> MRSSKSPFKRKSHSRETSHDENTSFFHKRTISGSSAHHSRNVSQGAVPSSAPPVSGGNYSHKRNVSRASNSSQTSNFLAEQYERDRKAIINCCFSRPDHKTGEPPNNYITHVRIIEDSKFPSSRPPPDSKLENKKKRLLILSAKPNNAKLIQIHKARENSDGSFQIGRTWQLTELVRVEKDLEISEGFILTMSKKYYWETNSAKERTVFIKSLITLYIQTFEGHVPELVNWDLSLFYLDERSYQRAVITNRPGSVSPIKSPTSNFTTNTTQSVGSVPFSAPTERTRRSETESVNPVSTPASVEYHAGMKSLNKAPYSSNSTLNEVNKRYELEQQQQQEEAELRRLEEQKRLQLQKENEMKRLEEERRIKQEERKRQMELEHQRQLEEEERKRQMELEAKKQMELKRQRQFEEEQRLKKERELLEIQRKQREQETAERLKKEEQEALAKKEEEEKSKRNKVDNESYTQEINGKVDNLLEDLNAVLAEETETTPTMQNGTYVPERSTARAHDQLKKPLNIAKVESLGGSDLNDSISLSDEIAGLNTSNLSGEDQDEKNDLSFEKGDEVRYSNNFEGEAPHVYHEVSIIQEEAPAVSQKLILPEENNESEALIESKEEIKTMENIDDEVLLEILTDINWSIEDDADSMIERIDLRLAETEYLFNQNLLSLQKIGPNIRPYEDKVNDECHRIIPTLSLFLMEMSNFSNDIENVESQDNGLQVESANKKLLWNTLDELLKTVSLDEISLNQLLECPIREKNLPWMENQLNLLLKAFQAIGSDGNEVEYNLREISGLKQRLQFYEKVTKIFLNRIVEEMQKKFSNIRGQDISHDQMIRILTTLLIFSPLILFCKEISQKSYQAIVENWNVSIQPVYMELWTKKISQLQGIDTNDEKMNELSLSQLLNEWDTFRKERKTNDINPVFKNSFSLLTECLQTMRQECIVYQNFVEVFFHISSKHNFEEYIKHFNDPDAPPILLDTVKVMQSDREAAVIETQLVSRIFQPIVTRLSSYFVELVKAEPTVAPALTFYLENEIKSLESSNHEFLLSAVTRMYTQIKQVWSDNVEEQVLHFERISNATTNGEILPGILDLPVGLKNSEDLFQFAKRSMDIKDTDEGYESIELMNSSFRKLSIAATRSITHKEVNSSINPNLSDTAALNNDYMETISLLVNSNWLTEMLSMLNFNKDGIFDTSLQNVKKVFDVEKESYASFLLRDTMPKLTAFVYGVSNIIENTNNVNMTNPSRWAAYSRQNLENILLAYTSHEIETLVKRLHTHMVNDFGYHQENAINNVLCDKLWSCIQGQTVSLYLKLYTVIDKHYRGTNIRFTKNDIISAFEEYKNA;> MDRFQIGDEQLLRFYQLKTINPTHSWAQDSSKLNNEEATSNELGVETSFDILKDFKYGNQISIDKESRAYLNDESLSYIRDPLNGQEMSKELQHLPNDSMRLNYLVNSKQFNVKAFLRDMHKQDSFNDLNNSLDRLDSDIQDQSIHLKQLVGKNFTKYVKIKNKLDQIYKEFDEKTNEKNQCDSPKENQINVESLNKKVDEVIRTTTFKLKPLMDNYQKILNYQATKKFIELNKFYFNLPKSLKRCLTNNDFNEFIIEYSKGLTLRRRFNQSSDASQSLVIKRIWTQIENLLVTYKDLIWNSLINSNFNIDQPQETILSLFSKLLNLENFINNNQRESESGNKNTTSSSNENPILRWMSIKMNGFQNELNELSGHMISKIIHSQRLILQNNTNQDKSQGCVELSYYLKINQLFQIISDTGKDSEGLKSTVEPNKVNTISGTSYLNLNCQPSSQGLTDSPTIIEMWLLILKYINDLWKICDQFIEFWEHIEKFLDGTYQNSIINEKRKENILIGDSNIIESYQKSLILKEEQINEVRLKGEEFITSVSQNLISFFTSSQSSLPSSLKDSTGDITRSNKDSGSPLDYGFIPPNCNGLSCLRYLPKIVEPILKFSTELAQLNITTNGITICRNTLSTIINRCVGAISSTKLRDISNFYQLENWQVYETVTFSSKSQDSSKNLTFEYGVTQFPEIVTSFQEVSIKTTRDLLFAYEKLPIINGISVVSYPSKQLLTGIEIQQIISMEAVLEAILKNAAKDKDNPRNSHTILTLTNLQYFRECAFPNILQYFDDAFEWNLASKNLELFSLLSKMESSIFGNYLSDLKINLRDTLEEKFHEINWPMYTSNSFRVGDYIIEALMILIVVHSECFRIGPQLIHKILIETQIFIARYLFEAFKPYVGNLSNDGSLQIIVDLEFFQKVMGPLLEKDTEATLRACLQNCFQNDTNRLQKCINEINPIVSANLKRTAIQFAAFS;> MSSDPLQQVCDLIKGDLSLERVRDIKEQLLKEKSVVEYQLNKESDKYYGEVEESLKLLNLSKNSVTSIKQQINEVNKLGNDNRFAINRYDILFRATKLYETVNTTSSIYDRIYNFVALMEHIERLLVAELAEDALETGCPHLLEIHFLLTSARDFQEQVVVMAKEATEDAQRTVMKLFSRLSGIISKFDKLLDGLTYDIVEMARAEQISLAIRLFKIYDLEEREDLRIEAIRNIIKKKEIEIEKSSIKKLPNSKNTARLQDETPKVIEYPTNKGLYQEIMSGTISTRTAPRGYKHFLINGINNSISEMFGEMREKYVGDQKFDVLDNMDWIFNELIIVKEHIANCCPPHWNIFEVYFDQYYKELHSLITDLVESEPETIIILDILAFDKTFQDTLKQDFGFTKSEVKSVIGDKEKETLFKDYLNLIVVKMTEWIGNLEKAEFDVFLERSTPPHSDSDGLLFLDGTKTCFQMFTQQVEVAAGTNQAKILVGVVERFSDLLTKRQKNWISKISEEIKKQINYNHKYDIDPESITPEDECPGGLVEYLIAVSNDQMKAADYAVAISSKYGKLVSKVYEKQITNHLEGTLDGFAEVAQCSSLGLITLMFDDLRKPYQEIFSKTWYMGSQAQQIADTLDEYLLDIKPQMNSVLFVNFIDNVIGETIIKFLTALSFEHSFKNKNNKFLEAMKRDFEIFYQLFVKVLDGNESKDTLITQNFTVMEFFMDLSCEPIDSILDIWQKYLEVYWDSRIDLLVGILKCRKDVSSSERKKIVQQATEMLHEYRRNMEANGVDREPTLMRRFVLEFEKQ;> MDYLKPAQKGRRRGLSINSLSETQQSAMNSSLDHLQNDLNRINLQWNRILSDNTNPLELALAFLDDTSVGLGHRYEEFNQLKSQIGSHLQDVVNEHSQVFNTNVASYGKAVSSIMQAQEQTLNLKNCLKEANEKITTDKGSLQELNDNNLKYTKMIDVLVNIEELLQIPEKIEENIRKENFHQVQILLERGFILMNNKSLKTVEILKPINQQLELQEHLLFNNLIEEIHDIMYSKSNKTNFTRVTNNDIFKIISISHNGFTSLENYLYNIVNIDIMEHSKTINKNLEQFIHDQSLNKGNIMLQENAATQAPLAPSRNQENEGFNRIGFLLKTINNINKLPVAFNIITERAKEEIHNIIVKSTESIRSKHPSLLKMATSLKNDNHFGLPVQDILSIILRECFWEIFLKLLYAIQCHRAIFEMSNILQPTSSAKPAFKFNKIWGKLLDEIELLLVRYINDPELISSNNGSIKPINGATNNAPTLPKRKNPKIFSLEYNIEDNSSVKDQAFELKALLKDIFPGFSVSSNMDLDSIYVKDESFEQDEPLVPPSVFNMKVILDPFLLFTQSTSTIVPSVLTQNTISSLTFFDDYMNKSFLPKIQMTMDYLFTVEVESNNPYALELSDENHNIFKTALDFQRLFYNLLNVFNTANTFREKISYCILDLLNHFYNYYLGLFNSL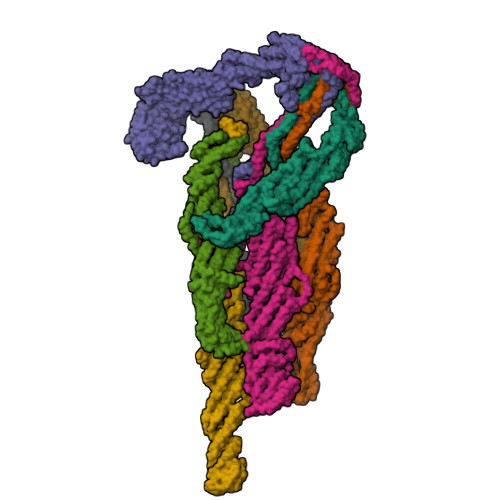IGTSDRHLTRKIITAWLQNGILMDQEQKILNGDETLFHEESIELFKEIPHFYQAGKGLSKSDLFNNLTLDTILQFSASVLWILNWLPGLKKAINIDEVSQEPMLDADRLRSSWTFSESMDLNYSNPSSSPNSLGNLKILLDDKASKKFDETIDGFKTLKFKLITILRFNIRALCIYDIGSFFQNTKIWNMDVGSIELDQNIASLISELRRTESKLKQQLPEKEKNSIFIGLDIVNNYALIKGAKSIKVLNHNGIKKMLRNVNVLQHAYRNLSSEPSKINMNVTMNFYSLCGSSEAELFEYIKDNELPHCSVEDLKTILRLQFSEEMHRQLKRQSTSSTKGSIKPSNKRYTEALEKLSNLEKEQSKEGARTKIGKLKSKLNAVHTANEK;> MNSLYELDPKWKKLLKTDNFLGGLTVNEFVQELSKDHRNDVLIDANTKNLPTNEKDQDAIREAIWKQLDPKPYIRTFESTLKELKNLNEETLNKRQYFSEQVATQEVIHSENVIKLSKDLHTTLLTFDKLDDRLTNVTQVVSPLGDKLETAIKKKQNYIQSVELIRRYNDFYSMGKSDIVEQLRLSKNWKLNLKSVKLMKNLLILSSKLETSSIPKTINTKLVIEKYSEMMENELLENFNSAYRENNFTKLNEIAIILNNFNGGVNVIQSFINQHDYFIDTKQIDLENEFENVFIKNVKFKEQLIDFENHSVIIETSMQNLINDVETVIKNESKIVKRVFEEKATHVIQLFIQRVFAQKIEPRFEVLLRNSLSISNLAYVRILHGLFTLFGKFTKSLIDYFQLLEIDDSNQILSTTLEQCFADLFSHYLYDRSKYFGIEKRSLEAILVDMTSKFTVNYDKEINKRVLLDKYKEKLSTNVDAFMHSPRGNTHSRQDSTSRSKLSQFNSFLKTHLDKDHLSLNRTNTLSDSFNNSSSSTQYDVANNSSSLVNSSFTASDIDNSPNSPANYSLNDVDSMLKCVVESTARVMELIPNKAHLYILEILKIMFLGIVDSYMEIALEVAYWKICKVDINKTAGVVNLNFLKFISMSTEILDLLSISIKSIFLPLLNNSPEIKAQIIEMTNSQIQKMEILINIILQETITVISTKFSAILCKQKKKDFVPKSQELLDQDTLPAIEIVNILNLIFEQSSKFLKGKNLQTFLTLIGEELYGLLLSHYSHFQVNSIGGVVVTKDIIGYQTAIEDWGVASLIDKFATLRELANLFTVQPELLESLTKEGHLADIGRDIIQSYISNREDFNHDNFINSVKLNFR;> MDQEGQPLLSKDFQQVLLATASGNNSSWTERAVLNNESTDAVKHEPALGQNDVFDLDPLSFDKWVPFLRRALDKNQLDPVIDELENSIEDNFQGLELQLLQDSQMNDKLETSIDEIANIQGMVQDTLSSEISKFQIRLSESANELIVKKQMYVNNKKISLKISEATILITKVVRILELSSKCQELITERKFFKVLQNLDSLEKLYLQEFKNYNFQFLIEIYNSIPFLQKVTKDECINLIRNSLNLNLGKNLIKVGQEFVAIYENELLPQWLETRSKMKLTNFKFNSPIEISMRDESFLAKLNLGEFFQLDDFHDSIMIFQNLNELSVLSGEFNKEYELRKTKLMYPLIWKKNKTAAYQMDSLLRGTGTTPGSTAHDVSTDDPFTQSLSLHFLQDYFLKILGFLLYDINLNKATEFILVDNNYNSTNEFWDGLMDRLSPYLSYFIDEKLKTEEDMIKLKDFLCIYVAILENFKLNIEPLYKILVSIFEKFCSVSLRAFDDEFQILLNDDDFMPLSINDKTLYEKVLKICWMKEGEHLSLPDPTNGEPFAVTLPFSPLYPMTCTLAKKTYSKITAFLSIFYRHELHTLNNILVKTMDDIFNDIVNKKIRSKLESTSREEIAQILVNLDYFIIAAKEFSNFMTRENILQNPDMEIRLSSIKYLAESRKLAETKLIELIDSKISDILETIEIDWQITEVRQDPDISIIDLAQFLEMMFASTLQNLPYSVQTLLIFREFDSLTRQFMGLLLHDTPSTITHESIMNFEVDVNYLESIIPRIFPSTPGTIDSNGYQSPMTPSTPTFPNANGVDAPTLFENNIKSLEATFMELKQCIELLKTQGKDYNEPEIRLRKYSRIRQEDAALLLSKIQHFVSSVEGANGDDTSVMDSSSIFNSESASVIDSNTSRIAKFFNRR;> MPAEIDIDEADVLVLSQELQKTSKLTFEINKSLKKIAATSNQSSQLFTPILARNNVLTTLQRNIESTLNSVASVKDLANEASKYEIILQKGINQVGLKQYTQVVHKLDDMLEDIQSGQANREENSEFHGILTHLEQLIKRSEAQLRVYFISILNSIKPFDPQINITKKMPFPYYEDQQLGALSWILDYFHGNSEGSIIQDILVGERSKLILKCMAFLEPFAKEISTAKNAPYEKGSSGMNSYTEALLGFIANEKSLVDDLYSQYTESKPHVLSQILSPLISAYAKLFGANLKIVRSNLENFGFFSFELVESINDVKKSLRGKELQNYNLLQDCTQEVRQVTQSLFRDAIDRIIKKANSISTIPSNNGVTEATVDTMSRLRKFSEYKNGCLGAMDNITRENWLPSNYKEKEYTLQNEALNWEDHNVLLSCFISDCIDTLAVNLERKAQIALMPNQEPDVANPNSSKNKHKQRIGFFILMNLTLVEQIVEKSELNLMLAGEGHSRLERLKKRYISYMVSDWRDLTANLMDSVFIDSSGKKSKDKEQIKEKFRKFNEGFEDLVSKTKQYKLSDPSLKVTLKSEIISLVMPMYERFYSRYKDSFKNPRKHIKYTPDELTTVLNQLVR;> MVEFSLKKARNNWKHVKKSASSPAKQKTPPSPAKPKQKTKKNPYSDLKDPATSYTLPTINARERSRVATSMQRRLSIHNTNYAPPTLDYSMPLPDMPNMIVPNDNVDSSHNNSSFTTENESVSSKGPSNSLNLSTADLSLNDSSYNKVPARSAMRNTVNPSGSNDPFNNSTSLRKMLANPHFNAKDFVHDKLGNASAITIDKFTSNLTDLSIQVQEEVKLNINKSYNEIMTVNNDLNVAMLELKRVRANINDLNEVLDQCTKIAEKRLQLQDQIDQERQGNFNNVESHSNSPALLPPLKAGQNGNLMRRDRSSVLILEKFWDTELDQLFKNVEGAQKFINSTKGRHILMNSANWMELNTTTGKPLQMVQIFILNDLVLIADKSRDKQNDFIVSQCYPLKDVTVTQEEFSTKRLLFKFSNSNSSLYECRDADECSRLLDVIRKAKDDLCDIFHVEEENSKRIRESFRYLQSTQQTPGRENNRSPNKNKRRSMGGSITPGRNVTGAMDQYLLQNLTLSMHSRPRSRDMSSTAQRLKFLDEGVEEIDIELARLRFESAVETLLDIESQLEDLSERISDEELMLLNLISLKIEQRREAISSKLSQSILSSNEIVHLKSGTENMIKLGLPEQALDLFLQNRSNFIQDLILQIGSVDNPTNYLTQLAVIRFQTIKKTVEDFQDIFKELGAKISSILVDWCSDEVDNHFKLIDKQLLNDEMLSPGSIKSSRKQIDGLKAVGLDFVYKLDEFIKKNSDKIR>MATSLNTIDIQGDILVGMHKQKQLFYFFAINDPATFKTHLASDIAPVVASVTQLSNVATQPLVALNIAFSNTGLLALGVTDNLGDSLFANGQAKDATSFKESTSSWVPQFAGTGIHGVIILASDTTDLIDQQVASIESTFGSSISKLSSLSASIRPGNEAGHEMFGFLDGIAQPAINGFNTPLPGQNIVDAGVIITGATNDPITRPSWAVGGSFLAFRQLEQLVPEFNKYLLDNAPAGSGSLQARADLLGARMVGRWKSGAPIDLTPTADDPALGADAQRNNNFTYSHAGFDLGSDQSHCPFSAHIRKTRPRADLGGSLTPPNLSAGANSIMRSGIPYGPEVTSAESASNTTTQERGLAFVAYQAQLSQGFHFLQQTWADNANFPPGKTPATVGLDPIIGQNN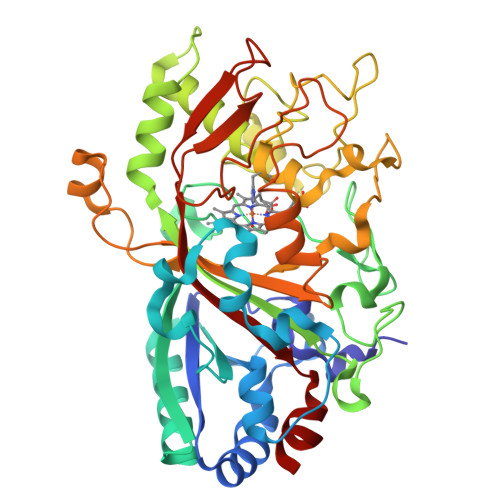GQPRVVNGLLPSNSSASLSIPQFVVSHGGEYFFSPPISAIGGRLSA[2x]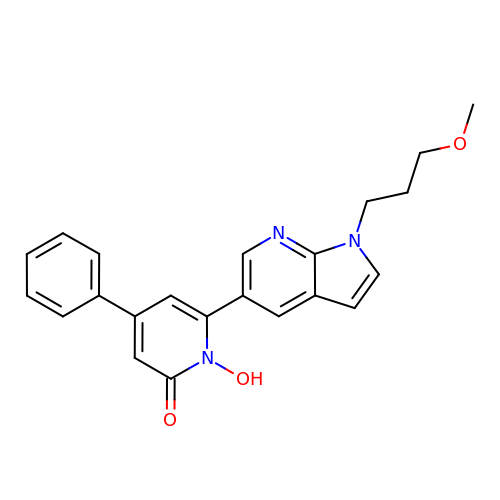1-hydroxy-6-[1-(3-methoxypropyl)-1H-pyrrolo[2,3-b]pyridin-5-yl]-4-phenylpyridin-2(1H)-one | C22 H21 N3 O3 | MIWLVFZOCHMICD-UHFFFAOYSA-N>[2x]MAESLLIKDIAIVTENEVIKNGYVGINDGKISTVS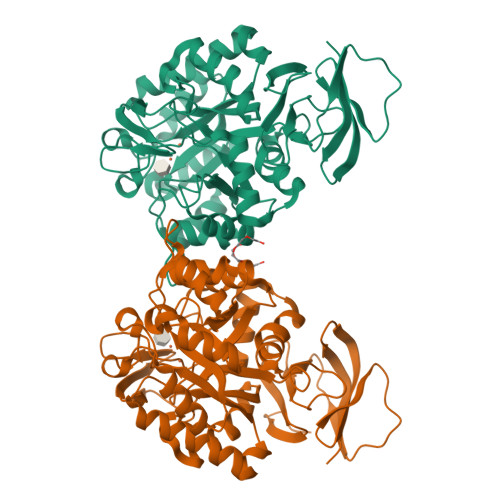TERPKEPYSKEIQAPADSVLLPGMIDIHIHGGYGADTMDASFSTLDIMSSRLPEEGTTSFLATTITQEHGNISQALVNAREWKAAEESSLLGAELLGIHLEGPFVSPKRAGAQPKEWIRPSDVELFKKWQQEAGGLIKIVTLAPEEDQHFELIRHLKDESIIASMGHTDADSALLSDAAKAGASHMTHLYNAMSPFHHREPGVIGTALAHDGFVTELIADGIHSHPLAAKLAFLAKGSSKLILITDSMRAKGLKDGVYEFGGQSVTVRGRTALLSDGTLAGSILKMNEGARHMREFTNCSWTDIANITSENAAKQLGIFDRKGSVTVGKDADLVIVSSDCEVILTICRGNIAFISKEADQI>CG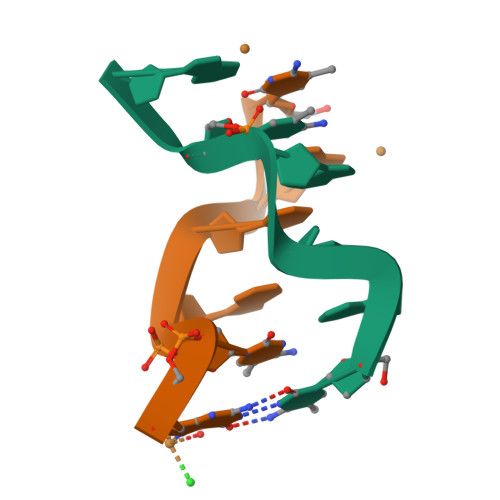UACG[2x]The BisI family of restriction endonucleases is unique in requiring multiple methylated or hydroxymethylated cytosine residues within a short recognition sequence (GCNGC), and in cleaving directly within this sequence, rather than at a distance. We present the crystal structures of NhoI and Eco15I_Ntd (N-terminal catalytic domain of Eco15I) in the absence of DNA and in specific complexes with fully methylated GCNGC containing dsDNA. Both proteins are homodimeric, with each domain involved in target sequence recognition and catalysis. The crystal structures show that the modified cytosine bases are recognized in the context of double-stranded DNA, without base flipping.

We truncated the enzyme to the shortest active form of the catalytic domain (containing 173 amino acids) to increase the quality of crystals and refer to this truncated form as Eco15I_Ntd. Crystals of NhoI and Eco15I_Ntd could be grown in the absence of DNA, and as specific complexes with tetra-methylated G5mCNG5mC DNA with Ca2+ cations replacing the Mg2+ cofactor. In the crystal structures of NhoI and Eco15I_Ntd with DNA, the dimerization and DNA binding modes are very similar. In the co-crystal structures with bound DNA, the channel is closed on top by the hairpins of β-strands β7 and β8. A single Ca2+ ion from the buffer is present in the active sites of NhoI and Eco15I_Ntd in complex with DNA. As expected, this Ca2+ ion is coordinated by the aspartate of PD and the glutamine of QVK. In the co-crystal structures of NhoI and Eco15I_Ntd with DNA, the internal methyl groups (G5mCNGC) interact with the side chains of an (H/R)(V/I/T/M) di-amino acid motif near the C-terminus of the distal enzyme subunit and arginine residue from the proximal subunit. The external methyl groups (GCNG5mC) interact with the proximal enzyme subunit, mostly through main chain contacts. All described interactions of NhoI with the internal methyl groups in DNA are conserved in the Eco15I_Ntd–DNA complex. Here, the relevant residues are His139 and Val140 from the distal subunit and Arg98 from the proximal subunit.

>[2x]GSSYDWLNALNNLELLSLHSEILTQLRSRGVIRTKNNPVGDYAEWLVSNALGMTLLSNSSAGADAIDADGLKVQIKARRVTPDNPSRQLSALRNYEAADFDYLIAVIFDETYNILDAYKIPHEVIRDYARHSDHVNAHIVNLKGAILTDPRVSSIKEDLIVRSSASVNEAAMQT> MNYKISEL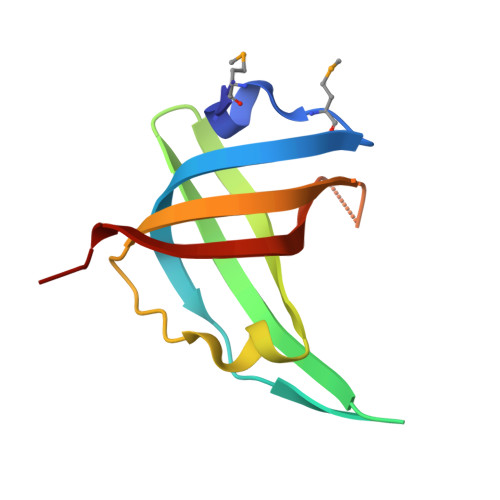MPNLSGTINAEVVTAYPKKEFSRKDGTKGQLKSLFLKDDTGSIRGTLWNELADFEVKKGDIAEVSGYVKQGYSGLEISVDNIGIIEKSL>[2x]PVFSADPGAPAPVNPCCYYPCQHQGICVRFGLDRYQCDCTRTGYSGPNCTIPEIWTWLRTTLRPSPSFIHFLLTHGRWLWDFVNATFIRDTLMRLVLTVRSNLIPSPPTYNIAHDYISWESFSNVSYYTRILPSVPRDCPTPMGTKGKKQLPDAEFLSRRFLLRRKFIPDPQGTNLMFAFFAQHFTHQFFKTSGKMGPGFTKALGHGVDLGHIYGDNLERQYQLRLFKDGKLKYQMLNGEVYPPSVEEAPVLMHYPRGIPPQSQMAVGQEVFGLLPGLMLYATIWLREHNRVC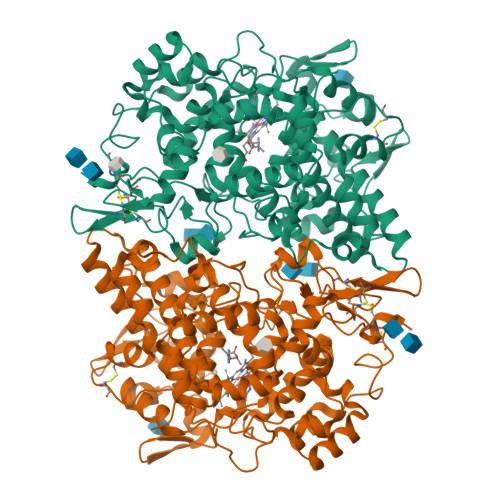DLLKAEHPTWGDEQLFQTARLILIGETIKIVIEEYVQQLSGYFLQLKFDPELLFGAQFQYRNRIAMEFNQLYHWHPLMPDSFRVGPQDYSYEQFLFNTSMLVDYGVEALVDAFSRQPAGRIGGGRNIDHHILHVAVDVIKESRVLRLQPFNEYRKRFGMKPYTSFQELTGEKEMAAELEELYGDIDALEFYPGLLLEKCHPNSIFGESMIEMGAPFSLKGLLGNPICSPEYWKASTFGGEVGFNLVKTATLKKLVCLNTKTCPYVSFHVPDPRQEDRPGVERPPTEL>[2x]MPNFSGNWKIIRSENFEELLKVLGVNVMLRKIAVAAASKPAVEIKQEGDTFYIKTSTTVRTTEINFKVGEEFEEQTVDGRPCKSLVKWESENKMVCEQKLLKGEGPKTSWTRELTNDGELILTMTADDVVCTRVYVRE

The cellular retinoic acid-binding proteins CRABPI and CRABPII act as gatekeepers and facilitators for the passage of all-trans-retinoic acid (and related derivatives) through the cytoplasm to access retinoic acid receptors (RARs) in the nucleus. In this article, crystal structures are presented of the L29C mutant of Homo sapiens CRABPI in complex with naturally occurring fatty acids (1.64 Å resolution) and with the synthetic retinoid DC645 (2.41 Å resolution), and of CRABPII in complex with the ligands DC479 (1.80 Å resolution) and DC645 (1.71 Å resolution). The retinoic acid-binding ability of both CRABPI and CRABPII is centred on a hydrophobic pocket created by an orthogonal β-sheet fold and capped with a pair of antiparallel α-helices formed from residues 15–35 partway into the sequence. The pocket contains, at its most buried end, a trio of residues (Arg112, Arg132 and Tyr134 in CRABPI; Arg112, Arg133 and Tyr135 in CRABPII) that are responsible for binding to the carboxylic acid moiety of ATRA, usually in concert with a water molecule that is conserved in all structures with similarly binding ligands.

Wild-type CRABPII expressed recombinantly in E. coli proved to be reliable for crystallization in a repeatable manner and accepted ligands for co-crystallization using an equimolar combining step prior to setting up crystallization drops. Seeking to identify ligands with unconventional binding-site interactions with CRABPII, DC479 was chosen from a number of small-molecule retinoids designed to substantially improve upon the intrinsic fluorescence of the retinoid family and particularly for use in high-throughput binding assays. Of particular interest was the extended carbon chain to which the carboxylic acid group was appended, improving the flexibility around the head group, to determine how ligand flexibility would affect optimum binding into the triad site. The compound binds to CRABPII with an affinity in the 50 nM range, similar to those of other ‘strongly binding’ synthetic derivatives, and thus was an ideal choice to explore ligand-conformation space in terms of interactions with the protein. Additionally, DC479 has been shown to cause the activation of nongenomic pathways whilst having no effect on genomic signalling; a result indicated by a lack of neurite outgrowth in tests with in vitro models. Indeed, its interactions with CRABPII may indicate why this is the case if the effect is caused by carrier-protein interactions rather than RAR binding (or a lack thereof) in the nucleus. DC479 occupies the binding site fully, with its carboxylic acid head buried adjacent to the canonical binding triad and conserved water molecule. Correct incorporation of the ligand suggests that it is not interaction with CRABPII that prevents genomic signalling in the case of DC479, which is discussed further below.[(1Z)-5-fluoro-2-methyl-1-{[4-(propan-2-yl)phenyl]methylidene}-1H-inden-3-yl]acetic acid | C22 H21 F 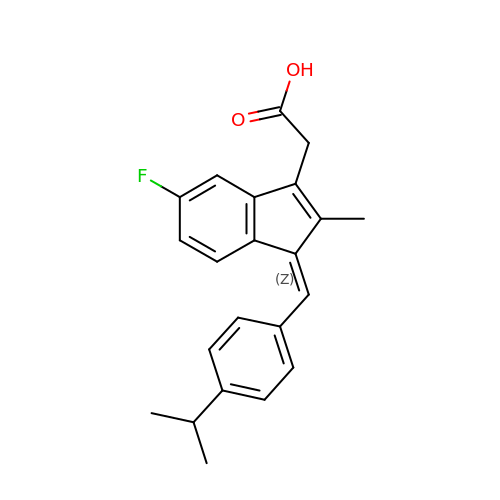O2 | QCXBVGNDRYQVJO-GRSHGNNSSA-N> MVRQYKIHTNLDGTDDKVWDVTNGKVRFYQPSNLGLQSTNNIWQSNGIGVMGTRSITQPQIEFKLETFGESLEENYQLMKDFVNDILSKKFVTLEYQTEIFQVYADLALADVTKTEGYGKNGTFSEKITFDIITKWYTYENLTFDKIQNGKVIAGMSKIYGGTAPGNYKYIKGTSYTYYGESDIDRLSRWDIKEEIFSFMGILYPKLPKTPAGVRFLDDIGNEYT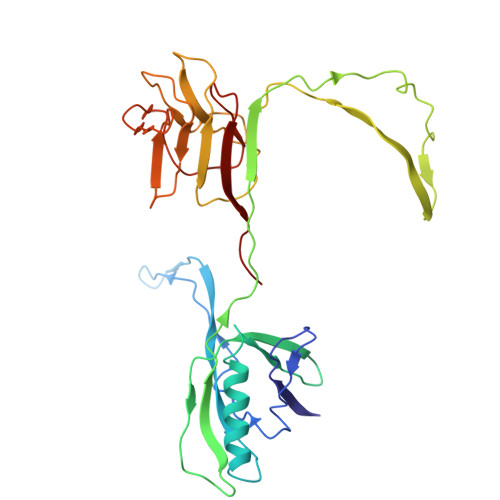AIVFKTEQVQDYILINTDVNDETYQGWKGTTALNLFPVMDFERYRTRIIEKGQMELINLSKAEFKIKRKADFV>[2x]QVTTEAPAKVVKHSKKQDENIVVNKFKPKEPYVGRCLLNTKITGDDAPGETWHMVFSTEGEVPYREGQSIGIVPDGIDKNGKPHKLRLYSIASSAIGDFGDSKTVSLCVKRLVYTNDAGEVVKGVCSNFLC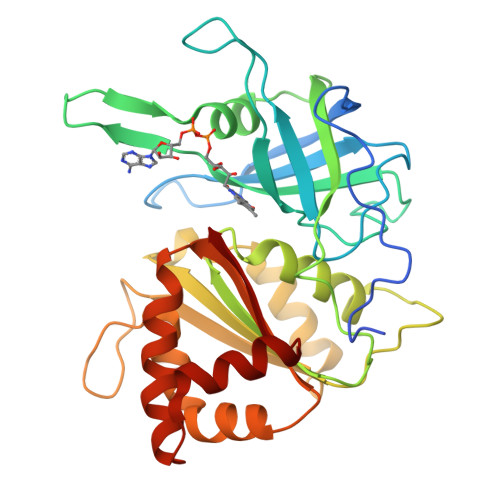DLKPGSEVKITGPVGKEMLMPKDPNATVIMLGTGTGIAPFRSFLWKMFFEKHEDYQFNGLAWLFLGVPTSSSLLYKEEFEKMKEKAPENFRLDFAVSREQVNDKGEKMYIQTRMAQYAEELWELLKKDNTFVYMCGLKGMEKGIDDIMVSLAAKDGIDWIEYKRTLKKAEQWNVEVY>[4x]MKKTKIVCTIGPKTESEEMLAKMLDAGMNVMRLNFSHGDYAEHGQRIQNLRNVMSKTGKTAAILLDTKGPEIRTMKLEGGNDVSLKAGQTFTFTTDKSVIGNSEMVAVTYEGFTTDLSVGNTVLVDDGLIGMEVTAIEGNKVICKVLNNGDLGENKGVNLPGVSIALPALAEKDKQDLIFGCEQGVDFVAASF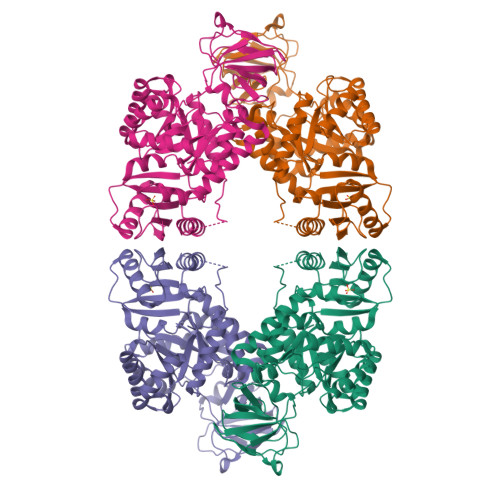IRKRSDVIEIREHLKAHGGENIHIISKIENQEGLNNFDEILEASDGIMVARGDLGVEIPVEEVIFAQKMMIEKCIRARKVVITATMMLDSMIKNPRPTDAEAGDVANAILDGTDAVMLSGESAKGKYPLEAVSIMATICERTDRVMNSRLEFNNDNRKLRITEAVCRGAVETAEKLDAPLIVVATQGGKSARAVRKYFPDATILALTTNEKTAHQLVLSKGVVPQLVKEITSTDDFYRLGKELALQSGLAHKGDVVVMVSGALVPSGTTNTASVHVL>[2x]MKGFFAGVVAAATLAVASAGDYCGQWDWAKSTNYIV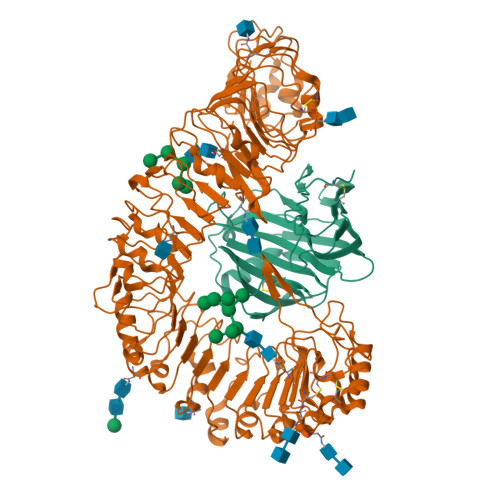YNNLWNKNAAASGSQCTGVDKISGSTIAWHTSYTWTGGAATEVKSYSNAALVFSKKQIKNIKSIPTKMKYSYSHSSGTFVADVSYDLFTSSTASGSNEYEIMIWLAAYGGAGPISSTGKAIATVTIGSNSFKLYKGPNGSTTVFSFVATKTITNFSADLQKFLSYLTKNQGLPSSQYLITLEAGTEPFVGTNAKMTVSSFSAAVN;>[2x]MGKREYPSSAHFLVTLSLLLLQAAFGLTLCIEKERDALLEFKRGLSDNFGQLSTWGDEEDKKECCKWKGIECNKTTGHVIVLDLHNAFTCSASACFAPRLTGKLSPSLLELEYLNFLDLSVNEFERSEIPRFICSFKRLEYLNLSSSFFSGLIPTQFKNLTSLRILDLGYNNLIVKDLTWLSHLSSLELLSLGGSDFQVKNWFQEITKLPLLKELDLSLCGLSKLVPSPAEIANSSLISLSVLHLCCNEFSSSAKYSWLFNFSTSLTSIDLSNNQLDGQIDDRFGNLMYLEHLNLANELNLKGGIPSSFGNLTRLRYLDMSNTRTYQWLPELFVRLSGSRKTLEVLGLNDNSMFGSLVDVTRFSALKRLYLQKNVLNGFFMERFGQVSSLEYLDLSDNQMRGPLPDLALFPSLRELHLGSNHFNGRIPQGIGKLSQLKILDVSSNRLEGLPESMGQLSNLESFDASYNVLKGTITESHLSNLSSLVDLDLSFNSLALKTSIDWLPPFQLQVINLPSCNLGPSFPKWLQSQNNYTVLDISLANISDALPSWFSGLPPDIKILNLSNNQISGRVSDLIENAYDYMVIDLSSNNFSGPLPLVPTNVQIFYLHKNQFFGSISSICKSTTGATSLDLSHNQFSGELPDCWMNATNLAVLNLAYNNFSGKLPQSLGSLTNLEALYMRQNSFSGMLPSLSQCQSLQILDLGGNKLTGRIPAWIGTDLLNLRILSLRFNKFYGSISPIICQLQFLQILDLSANGLAGKIPQCFNNFTLLHQENGLGEPMEFLVQGFYGKYPRHYSYLGNLLVQWKNQEAEYKNPLTYLKTIDLSSNKLVGGIPKEMAEMRGLKSLNLSRNDLNGSIIKGIGQMKMLESLDLSRNQLSGMIPKDLANLTFIGVLDLSNNHLSGRIPSSTQLQTFERSSYSGNAQLCGPPLQEC> GSALSEI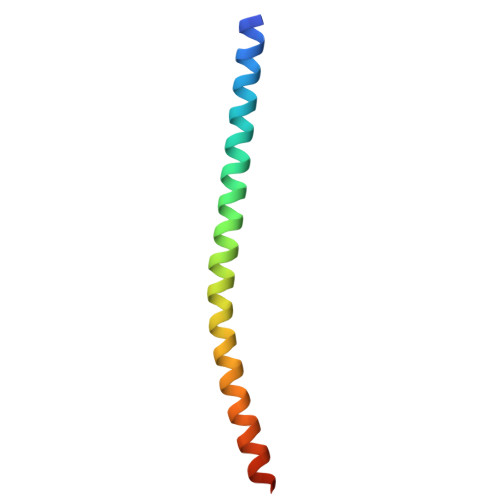ETRHSEIIKLENSIRELHDMFMDMAMLVESQGEMIDRIEYNVEHAVDYVERAVSDTKK>MHHHHHHDAMVKYEELLKTLENGINSEEGEIRLVRKSQGRFKEEFNFDLSLGSKPLLTLKVFLGRKPYWQPWVEVFGVNPNLRNVFFGS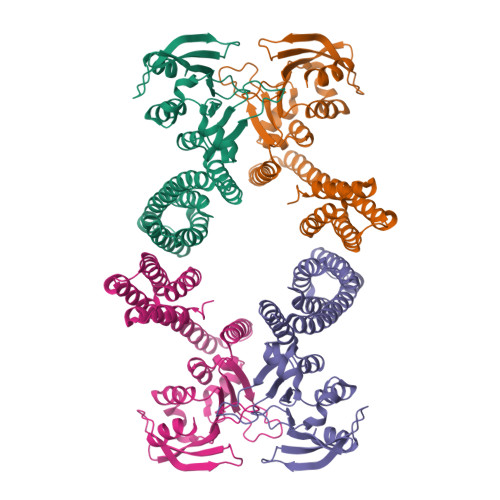EAERKLYEFLSEHFGRIFVEYFEDKETTYELQKGVPPALSRLGFELLKLGYTYFRDWFIPEGLMEGGHKIQAEKPKTAEAKARHLANLKKEFEEFIGKCEDEGLIKKVKERYNFLEEEAEERCRLAAQACIRACERYLALCTESSREQRQHAGDCADLCRLAALLLERRSPWAPAACELAARYALACAERCDGDEPLERECAGACRRFVAACAPLL[2x]>[3x]MGETKVIYHLDEEETPDLVKIPVPAERITLGDFKSVLQRPA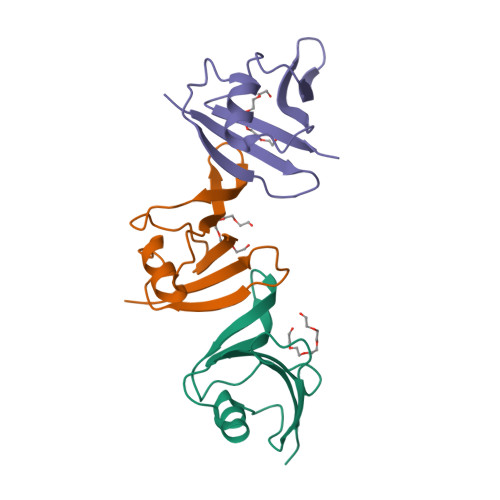GAKYFFKSMDQDFGVVKEEISDDNARLPCFNGRVVSWLVSSDNPQPEMAPPVHEPR> CGGPFELWEPNTTFSSTNFPNSYPNLAFCVWILNAQKGKNIQLHFQEFDLENINDVVEIRDGEEADSLLLAVYTGPGPVKDVFSTTNRMTVLLITNDVLARGGFKANFTTGYHLGIPEPCKADHFQCKNGECVPLVNLCDGHLHCEDGSDEADCVRFFNGTTNNNGLVRFRIQSIWHTACAENWTTQISNDVCQLLGLGSGNSSKPIFPTDGGPFVKLNTAPDGHLILTPSQQCLQDSLIRLQCNHKSCGKKLAAQDITPK;> IVGGSNAKEGAWPWVVGLYYGGRLLCGASLVSSDWLVSAAACVYGRNLEPSKWTAILGLHMKSNLTSPQTVPRLIDEIVINPHYNRRRKDNAIAMMHLEFKVNYTDYIQPICLPEENQVFPPGRNCSIAGWGTVVYQGTTANILQEADVPLLSNERCQQQMPEYNITENMICAGYEEGGIDSCQGDAGGPLMCQENNRWFLAGVTSFGYKCALPNRPGVYARVSRFTEWIQ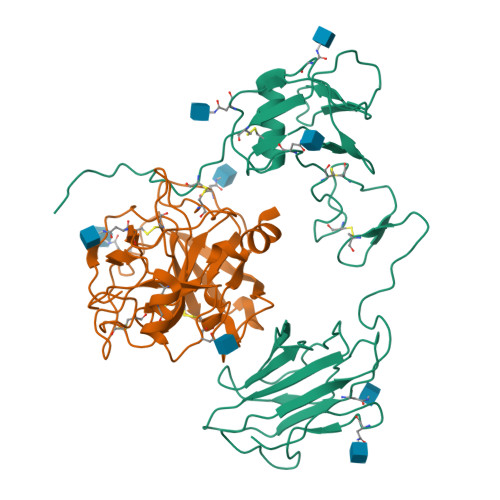SFLH> XQL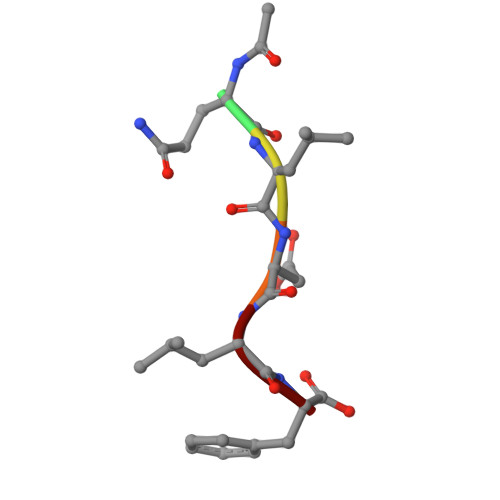DLF ABCB10, a member of ABC transporter superfamily that locates in the inner membrane of mitochondria, plays crucial roles in hemoglobin synthesis, antioxidative stress and stabilization of the iron transporter mitoferrin-1. Recently, it was found that ABCB10 is a mitochondrial biliverdin exporter. Each monomer contains two parts, the transmembrane domains (TMDs) and the nucleotide binding domains (NBDs). Here we report the cryo-EM structures of ABCB10 in apo (ABCB10-apo) and biliverdin-bound form (ABCB10-BV) at 3.67 Å and 2.85 Å resolution, respectively.

To determine the BV-bound ABCB10 structure, hopefully in outward-facing conformation, to uncover the molecular mechanism of BV export, ABCB10 E659Q mutant protein was vitrified in the presence of 1 mM BV. ABCB10-BV exhibits inverted V-shape homodimer and inward-facing conformation as well. The ABCB10 full transporter binds two BV molecules simultaneously. Each BV molecule is sandwiched at the interface of two protomers. TMH1-2 from one protomer and TMH4-6 from the opposing one form a pocket for one substrate. Indeed, the interactions between BV and ABCB10 can be divided into two parts: The hydrophobic interaction with one protomer and the hydrogen bond interaction with the other. BV contacts with residues on TMH4 (V322, V325, S326 and A329), TMH5 (F398, F399, T402, S405, N407, I409, and V410) and TMH6 (F439 and I443) hydrophobically. Two residues from the opposing protomer, namely S185 on TMH1 and N229 on TMH2, form hydrogen bonds with two carboxyl groups of BV. Binding with BV bring the two NBD close to about 13 Å. During the model building process, we unexpectedly noticed that two cholesterol molecules are sandwiched between two BVs.

> MAGLPEARKLLGLAYPERRRLAAAVGFLTMSSVISMSAPFFLGKIIDVIYTNPTVDYSDNLTRLCLGLSAVFLCGAAANAIRVYLMQTSGQRIVNRLRTSLFSSILRQEVAFFDKTRTGELINRLSSDTALLGRSVTENLSDGLRAGAQASVGISMMFFVSPNLATFVLSVVPPVSIIAVIYGRYLRKLTKVTQDSLAQATQLAEERIGNVRTVRAFGKEMTEIEKYASKVDHVMQLARKEAFARAGFFGATGLSGNLIVLSVLYKGGLLMGSAHMTVGELSSFLMYAFWVGISIGGLSSFYSELMKGLGAGGRLWELLEREPKLPFNEGVILNEKSFQGALEFKNVHFAYPARPEVPIFQDFSLSIPSGSVTALVGPSGSGKSTVLSLLLRLYDPASGTISLDGHDIRQLNPVWLRSKIGTVSQEPILFSCSIAENIAYGADDPSSVTAEEIQRVAEVANAVAFIRNFPQGFNTVVGEKGVLLSGGQKQRIAIARALLKNPKILLLDQATSALDAENEYLVQEALDRLMDGRTVLVIAHRLSTIKNANMVAVLDQGKITEYGKHEELLSKPNGIYRKLMNKQSFISAENLYFQGDYKDDDDKHHHHHHHHHH>HMSSGNASWFQAIKAKKLNTPPPKFEGSGVPDNENMKPSQQHGYWRRQARFKPGKGGRCPVPDAWYFYYTGTGPAADMNWGDTQDGIVWMA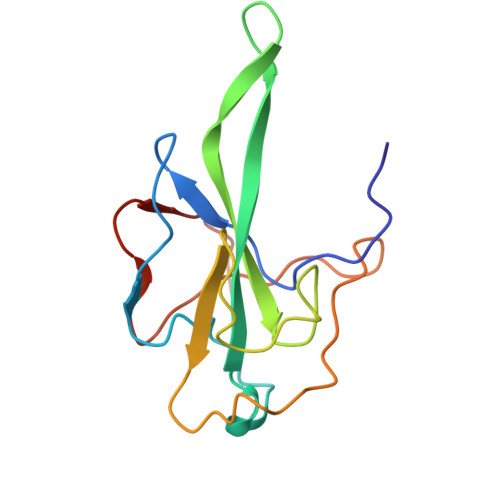AKGADTKSRSNQGTRDPDKFDQYPLRFSDGGPDGNFRWDFIPL[2x]5-(2-FORMYLTHIEN-5-YL)-URIDINE-5'-DIPHOSPHATE-ALPHA-D-GALACTOSE 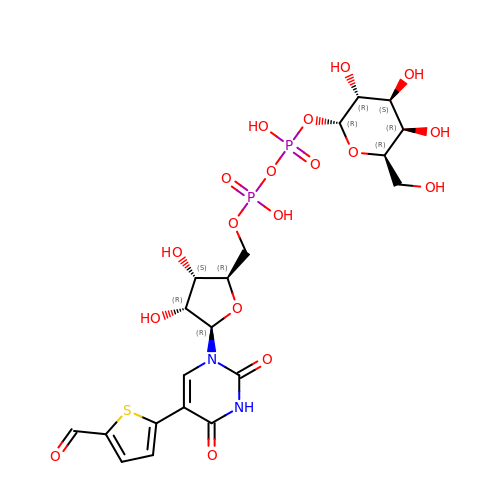| C20 H26 N2 O18 P2 S | KKHANSZRQMPJKN-PCGMDOMSSA-N>[2x]GGAKPLTDQEKRRQISIRGIVGVENVAELKKSFNRHLHFTLVKDRNVATTRDYYFALAHTVRDHLVGRWIRTQQHYYDKCPKRVYYLSLEFYMGRTLQNTMINLGLQNACDEAIYQLGLDIEELEEIEEDAGLGNGGLGRLAACFLDSMATLGLAAYGYGIRYEYGIFNQKIRDGWQVEEADDWLRYGNPWEKSRPEFMLPVHFYGKVEHTNTGTKWIDTQVVLALPYDTPVPGYMNNTVNTMRLWSARAPNDFNLRDFNVGDYIQAVLDRNLAENISRVLYPNDNFFEGKELRLKQEYFVVAATLQDIIRRFKASKFGSTRGAGTVFDAFPDQVAIQLNDTHPALAIPELMRIFVDIEKLPWSKAWELTQKTFAYTNHTVLPEALERWPVDLVEKLLPRHLEIIYEINQKHLDRIVALFPKDVDRLRRMSLIEEEGSKRINMAHLCIVGSHAVNGVAKIHSDIVKTKVFKDFSELEPDKFQ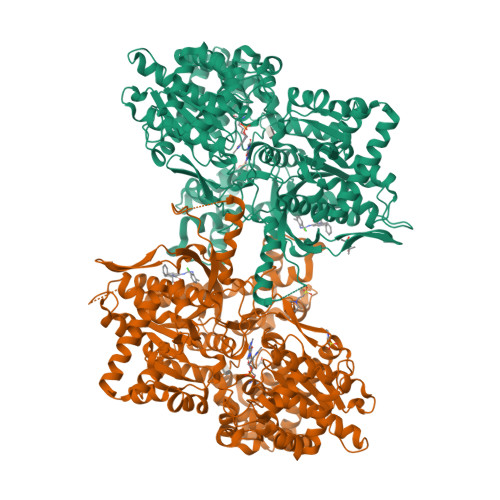NKTNGITPRRWLLLCNPGLAELIAEKIGEDYVKDLSQLTKLHSFLGDDVFLRELAKVKQENKLKFSQFLETEYKVKINPSSMFDVQVKRIHEYKRQLLNCLHVITMYNRIKKDPKKLFVPRTVIIGGKAAPGYHMAKMIIKLITSVADVVNNDPMVGSKLKVIFLENYRVSLAEKVIPATDLSEQISTAGTEASGTGNMKFMLNGALTIGTMDGANVEMAEEAGEENLFIFGMRIDDVAALDKKGYEAKEYYEALPELKLVIDQIDNGFFSPKQPDLFKDIINMLFYHDRFKVFADYEAYVKCQDKVSQLYMNPKAWNTMVLKNIAASGKFSSDRTIKEYAQNIWNVEPSDLKISLSNESNKVNGN1-THIEN-3-YLMETHANAMINE | C5 H7 N S | 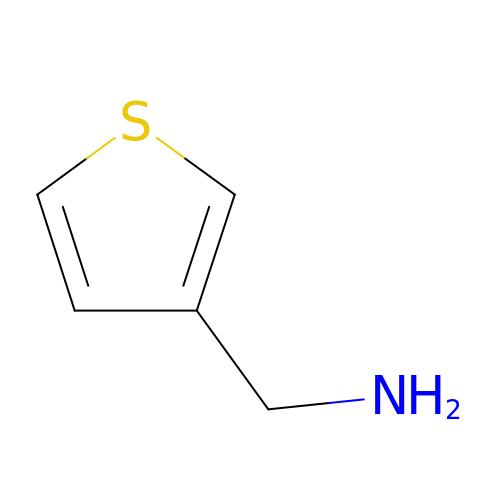DUDAKCCDHRNMDJ-UHFFFAOYSA-N>MGSSHHHHHHSSGRENLYFQGHERLTLDTRLRQALERNELVLHYQPIVELASGRIVGGEALV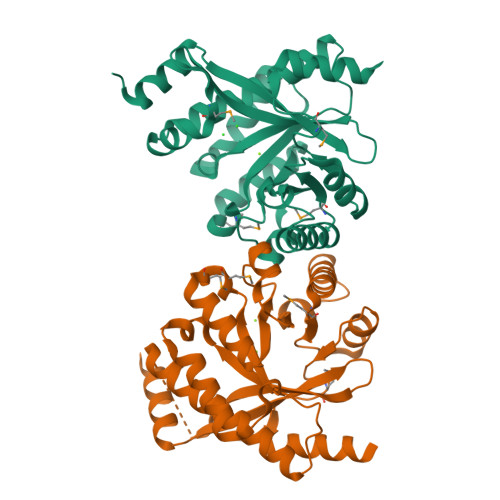RWEDPERGLVMPSAFIPAAEDTGLIVALSDWVLEACCTQLRAWQQQGRAADDLTLSVNISTRQFEGEHLTRAVDRALARSGLRPDCLELEITENVMLVMTDEVRTCLDALRARGVRLALDDFGTGYSSLSYLSQLPFHGLKIDQSFVRKIPAHPSETQIVTTILALARGLGMEVVAEGIETAQQYAFLRDRGCEFGQGNLMSTPQAADAFASLLDRQKASGQRPVHGHETAP[2x]>[2x]SNAQLDQIKARGELRVSTISSPLIYSTEKDTPSGFDYELAKRFADYLGVKLVIIPHHNIDDLFDALDNDDTDLLAAGLIYNR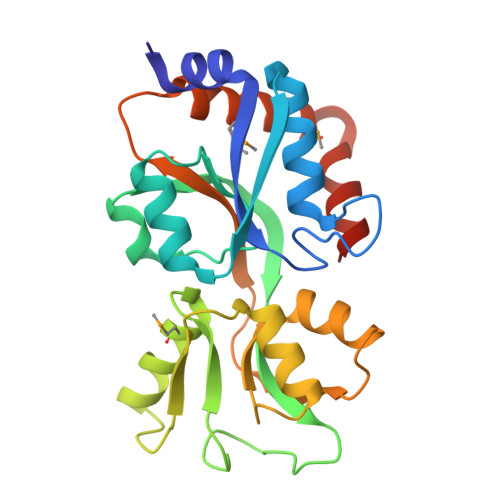ERLNRARTGPAYYSVSQQLVYRLGSPRPKSFSDLKGQVVVASGSAHMTTLKRLKQTKYPELNWSSSVDKSGKELLEQVAEGKLDYTLGDSATIALLQRIHPQLAVAFDVTDEEPVTWYFKQSDDDSLYAAMLDFYSEMVEDGSLARLEEKYLGHVGSFDYV THIAMIN PHOSPHATE | C12 H18 N4 O4 P S | 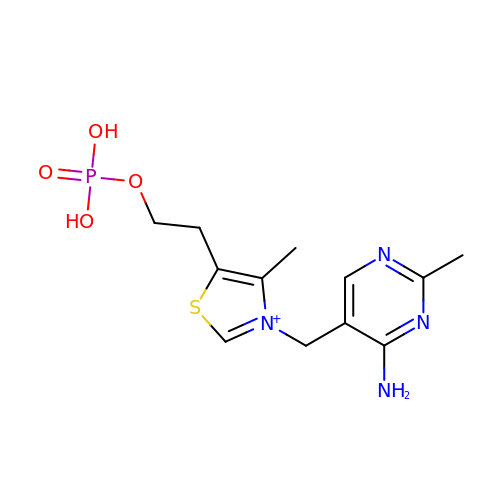HZSAJDVWZRBGIF-UHFFFAOYSA-O>MAQFDTEYQRLEASYSDSPPGEEDLLVHVAEGSKSPWHHIENLDLFFSRVYNLHQKNGFTCMLIGEIFELMQFLFVVAFTTFLVSCVDYDILFANKMVNHSLHPTEPVKVTLPDAFLPAQVCSARIQENGSLITILVIAGVFWIHRLIKFIYNICCYWEIHSFYLHALRIPMSALPYCTWQEVQARIVQTQKEHQICIHKRELTELDIYHRILRFQNYMVALVNKSLLPLRFRLPGLGEAVFFTRGLKYNFELILFWGPGSLFLNEWSLKAEYKRGGQRLELAQRLSNRILWIGIANFLLCPLILIWQILYAFFSYAEVLKREPGALGARCWSLYGRCYLRHFNELEHELQSRLNRGYKPASKYMNCFLSPLLTLLAKNGAFFAGSILAVLIALTIYDEDVLA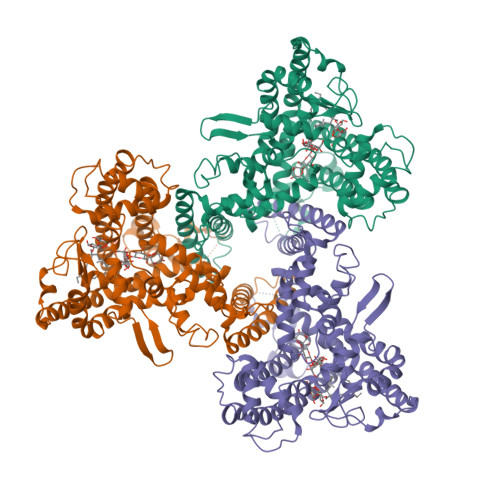VEHVLTTVTLLGVTVTVCRSFIPDQHMVFCPEQLLRVILAHIHYMPDHWQGNAHRSQTRDEFAQLFQYKAVFILEELLSPIVTPLILIFCLRPRALEIIDFFRNFTVEVVGVGDTCSFAQMDVRQHGHPQWLSAGQTEASVYQQAEDGKTELSLMHFAITNPGWQPPRESTAFLGFLKEQVQRDGAAASLAQGGLLPENALFTSIQSLQSESEPLSLIANVVAGSSCRGPPLPRDLQGSRHRAEVASALRSFSPLQPGQAPTGRAHSTMTGSGVDARTASSGSSVWEGQLQSLVLSEYASTEMSLHALYMHQLHKQQAQAEPERHVWHRRESDESGESAPDEGGEGARAPQSIPRSASYPCAAPRPGAPETTALHGGFQRRYGGITDPGTVPRVPSHFSRLPLGGWAEDGQSASRHPEPVPEEGSEDELPPQVHKV[3x]>[2x]DHYNCVSSGGACL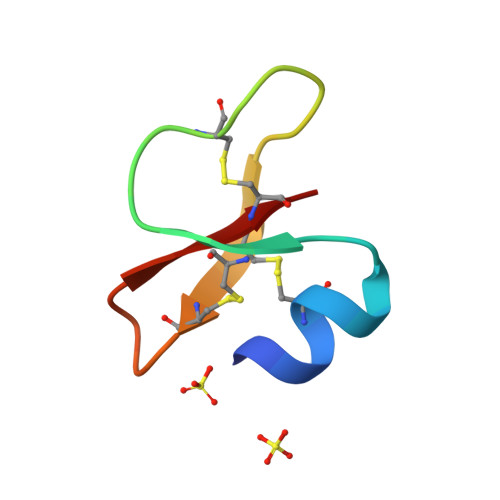YSACPIFTKIQGTCYRGKAKCCK>[4x]SNATRDALLKAMQVGETSIEAAEYMATRFEQILTK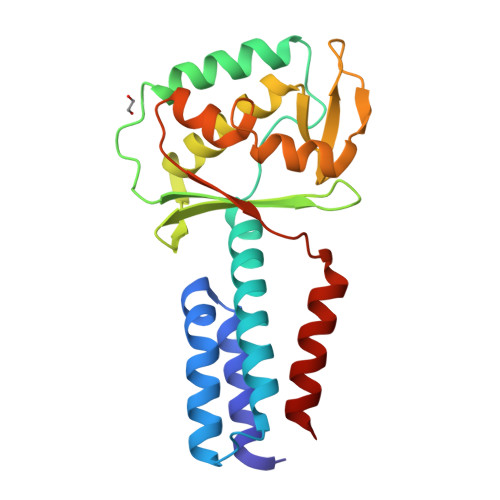AKLLPECNDMLEKIKEYAQFVKFKLLSSAQVWSGQERPTSDYQNTQENKAEFLASHLEGLPSGLKLEVAIGDDAKILRGFSSNGKMVEGDQLKTMDGLLEGWLAKNSLAISGGAVVKIDNTGNQTKVDPQEIRQLINDSEKGVAKYFADKGVGMEVAQRTYQEPKALETKREEIRQEIES>MVAPVSKNIGFLFLELRLDSKQQQIMDLVLKGVNAVMDTHHRNSFEPLHRGKFGAMKPLHVSLSETMMFANESELEEKMGRIRQEIRALECKSVPVALSGGWLVYENFDASLQFLAVGLSEPARGRLKPVLSIVEKYKP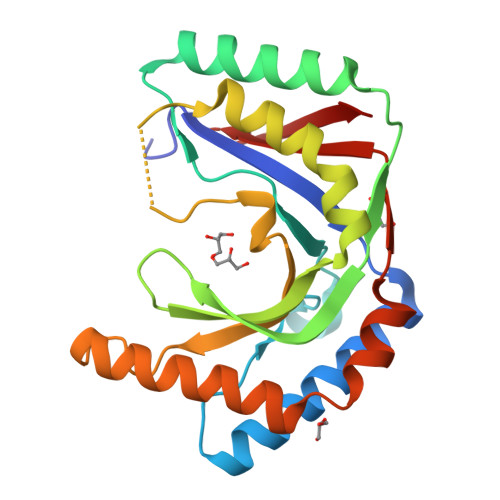RSPVSRQPVGLNNLHVSFGVAQNAYLQQDESVSRQRLDSLRNLVATEASDRLPLLRANLQFRCHELKAKVGTSVITLPL[3x]>MAHHHHHHVGTGSNDDDDKSPDPNWELVYTARLQMVKVLAVLYDGGEHAKQVPGLLGTTENELGLRKWLEDQGHTLVTTSDKDREGSTFDRELEDAEIIITTPFHPGYLTAERLARAKKLKLAVTAGIGSDHVDLDAANKTNGGITVAEVTGSCVVSVAEHVVMTILVLVRNFVPAHEQIEAGRWDVAEVAKDEYDLEGKVVGTVGVGRIGERVLRRLKGFDCKELLYYDYQPLSPEKEKEIGCRRVENLEEMLAQ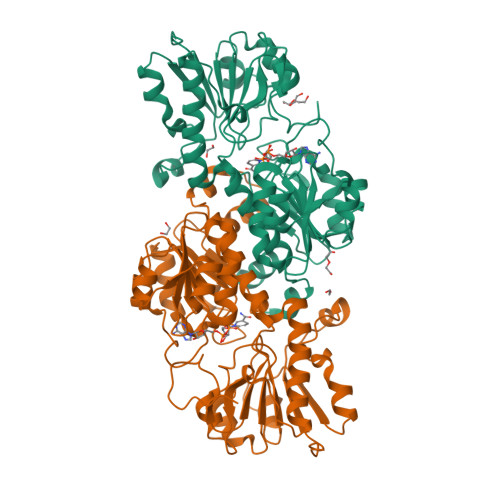CDVVTINCPLHESTRGLFNKDLISKMKRGSWLVNTARGAIVVKEDVAEALRTGHLRGYGGDVWFPQPAPADHVLRTAKNPFGGGNAMVPHMSGTSLDAQKRYAEGVKRILDSYLSGRFDYRPEDLIVHQGKYATRAYGQREDVKIPGQHHHHHH[4x]4-({4-[(2-fluorophenyl)amino]pyrimidin-2-yl}amino)benzoic acid | C17 H13 F N4 O2 | 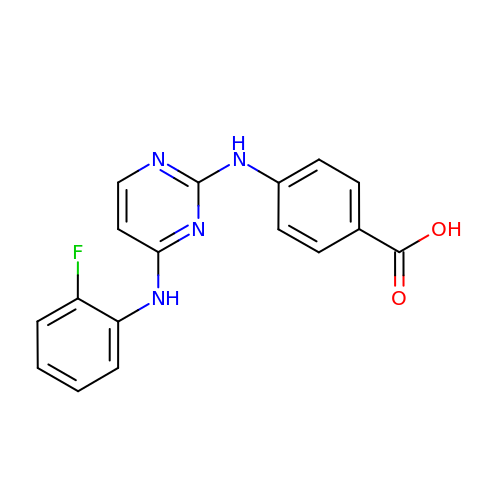DSRXYFSONVBAKS-UHFFFAOYSA-N> GPGSSLSRFRGCLAGALLGDCVGSFYAAHDTVDLTSVLRHVQSLEPDPGTPGSERTEALYYTDDTAMARALVQSLLAKEAFDEVDMAHRFAQEYKKDPDRGYGAGVVTVFKKLLNPKCRDVFEPARAQFNGKGSYGNGGAMRVAGISLAYSSVQDVQKFARLSAQLTHASSLGYNGAILQALAVHLALQGESSSEHFLKQLLGHMEDLEGDAQSVLDARELGMEERPYSSRLKKIGELLDQASVTREEVVSELGNGIAAFESVPTAIYCFLRCMEPDPEIPSAFNSLQRTLIYSISLG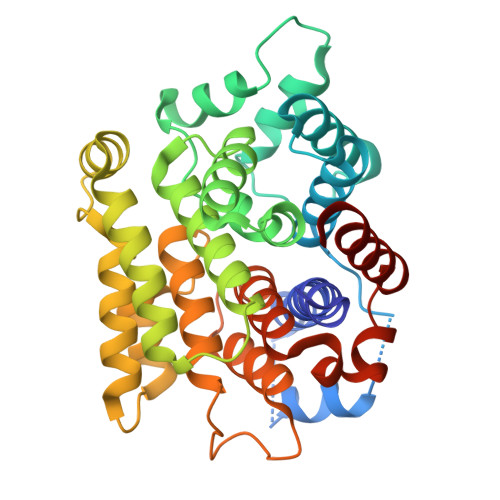GDTDTIATMAGAIAGAYYGMDQVPESWQQSCEGYEETDILAQSLHRVFQKS>[2x]MACALSVSGILCASQAATSFSSAKPTKSQPHPVQLKAFVPISQPAALKSASLVVSPSRTSHASVEAETEPFTLANIRESLIRQEDTIIYALLQRAQFSFNAPTYDENSFSIPGFKGSLVEFMLKETETLHAKVRRYQAPDEHPFFPEDLSQPILPSLPKSRVLHPAAEKININKSIWSMYLQDLLPKLTVPDDDGNYGSASVCDVLC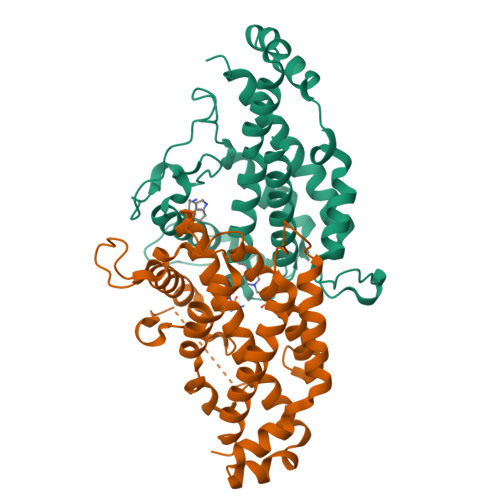LQALSKRIHYGKFVAEAKFIEDPARFEGHIKAQDGDAILRELTFKNVEDNVKRRVANKARAYGQEVNEHGKVDNARYKIDPDLAGALYEDWVMPLTKQVQVAYLLRRLD> HHHHSQDGGAYSDERQDLDQTIAEVSKELKLKLLIVENFIPRDVSERIKERAEWNEDSFEWNVNAFQSTSSNSSTPLNNTIEVNEDGVFTRSSGADSGVSVSGGNGTPATSQFLDKRLVATPGCRRPMSMCERMLVETAREQFGAQRRPPISGSGSFVEATIPEETIRFCGENVVVFSALERFVPEV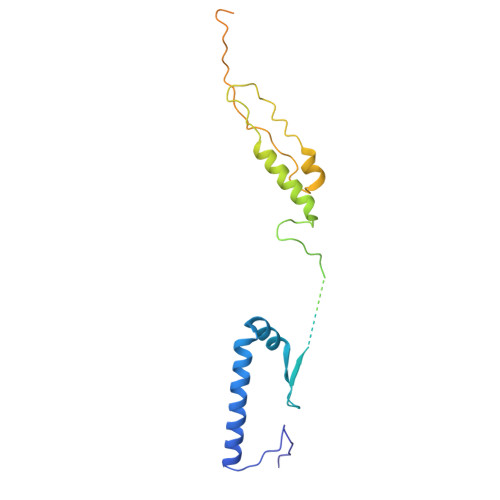TDSDPSTFSNSMMMSARRPSIENLTIDASKVLVPILNQSTMILKNSKNGQARNDTMPPNGSMRRSQN TMEM16K is a widely distributed, but relatively unstudied member of the TMEM16 family. Here we show that TMEM16K is an ER-resident lipid scramblase with non-specific ion channel activity and a dependence on calcium ions and short chain lipids for optimum activity. We present structures of TMEM16K solved by both X-ray crystallography and cryo-electron microscopy, revealing a classic scramblase fold, with extensive conformational changes propagated from the cytoplasmic to the ER face of the membrane, which lead to opening or closing of the lipid transporting groove. The TM domain of TMEM16K is C-terminal to the cytoplasmic domain and has ten TM α helices with TM3 to TM7 forming the lipid scramblase ‘groove’ and TM6 to TM8 forming the binding site for two Ca2+ ions, seen in other TMEM16s.

To understand whether TMEM16K can adopt alternative conformations and how changes in Ca2+ concentration affect the structure, we obtained three electron cryomicroscopy (cryo-EM) structures for TMEM16K in the presence of (i) 2 mM (‘high’) Ca2+, (ii) 430 nM (‘low’) Ca2+ and (iii) in the absence of Ca2+ (in 10 mM ethylene glycol-bis(β-aminoethyl ether)-N,N,N′,N′-tetraacetic acid (EGTA), ‘Ca2+-free’). These data sets had resolutions of 3.5, 4.2 and 5.1 Å respectively. The low and high Ca2+ structures are remarkably similar (mainchain r.m.s.d. of 0.42 Å); therefore below we describe the higher resolution 2 mM Ca2+ structure, unless otherwise stated. In the groove region, this conformation resembles the Ca2+-bound state of the mTMEM16A channel, and the recently published TMEM16F30, afTMEM1637 and nhTMEM1629 closed groove structures. The change from an open to a closed scramblase groove state is associated with extensive movements of the cytoplasmic domain and several transmembrane helices, leading to the ER end of the TM3−TM4 α-helical hairpin blocking the ER end of the groove. The closed scramblase groove has three distinct sections: a hydrophilic vestibule on the ER side of the membrane, a narrow neck and a cytoplasmic vestibule. The hydrophobic neck is lined with residues from TM4−7 (Tyr366, Ala367, Leu416, Ser415, Thr435, Leu436 and Tyr507), which together form a physical barrier to lipid movement. There is clear density for one complete lipid molecule in the 3.5 Å closed groove structure, lying adjacent to TM3, TM5 and TM9, in the cytoplasmic leaflet, a critical site for movement of the TM3−5 unit. The first unit rotates and moves up so that TM3−TM4 blocks the groove, while the second unit moves down, providing space for the first unit to rotate. These changes in TMEM16K conformation are not caused by changes in Ca2+ binding, as all three Ca2+-binding sites are occupied in both the 2 mM and 430 nM Ca2+ structures.

>MKVTLSALDTSESSFTPLVVIELAQDVKEETKEWLKNRIIAKKKDGGAQLLFRPLLNKYEQETLENQNLYLVGASKIRMLLGAEAVGLVKECNDNTMRAFTYRTRQNFKGFDDNNDDFLTMAECQFIIKHELENLRAKDEKMIPGYPQAKLYPGKSLLRRLLTSGIVIQVFPLHDSEALKKLEDTWYTRFALKYQPIDSIRGYFGETIALYFGFLEYFTFALIPMAVIGLPYYLFVWEDYDKYVIFASFNLIWSTVILELWKRGCANMTYRWGTLLMKRKFEEPRPGFHGVLGINSITGKEEPLYPSYKRQLRIYLVSLPFVCLCLYFSLYVMMIYFDMEVWALGLHENSGSEWTSVLLYVPSIIYAIVIEIMNRLYRYAAEFLTSWENHRLESAYQNHLILKVLVFNFLNCFASLFYIAFVLKDMKLLRQSLATLLITSQILNQIMESFLPYWLQRKHGVRVKRKVQALKADIDATLYEQVILEKEMGTYLGTFDDYLELFLQFGYVSLFSCVYPLAAAFAVLNNFTEVNSDALKMCRVFKRPFSEPSANIGVWQLAFETMSVISVVTNCALIGMSPQVNAVFPESKADLILIVVAVEHALLALKFILAFAIPDKPRHIQMKLARLEFESLEALKQQQMKLVTENLKEEPMESGKEKATAENLYFQ[2x]[[(2~{R},3~{S},4~{R},5~{R})-5-(2-azanyl-6-oxidanylidene-1~{H}-purin-9-yl)-3,4-bis(oxidanyl)oxolan-2-yl]methoxy-oxidanyl-phosphoryl] [[[(2~{R},3~{S},4~{R},5~{R})-5-(2-azanyl-6-oxidanylidene-1~{H}-purin-9-yl)-3,4-bis(oxidanyl)oxolan-2-yl]methoxy-oxidanyl-phosphoryl]oxy-oxidanyl-phosphoryl] hydrogen phosphate | C20 H28 N10 O21 P4 | 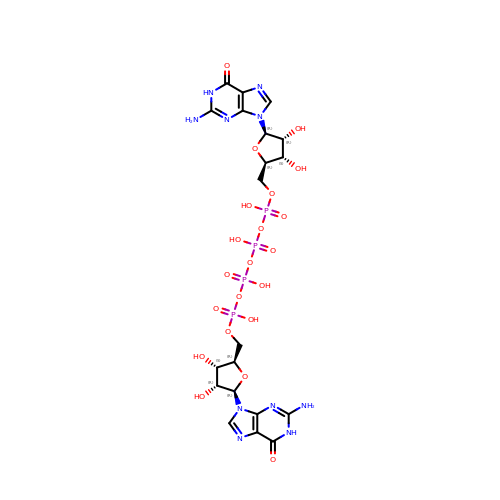OLGWXCQXRSSQPO-MHARETSRSA-N> MRIGIISVGPGNIMNLYRGVKRASENFEDVSIELVESPRNDLYDLLFIPGVGHFGEGMRRLRENDLIDFVRKHVEDERYVVGVCLGMQLLFEESEEA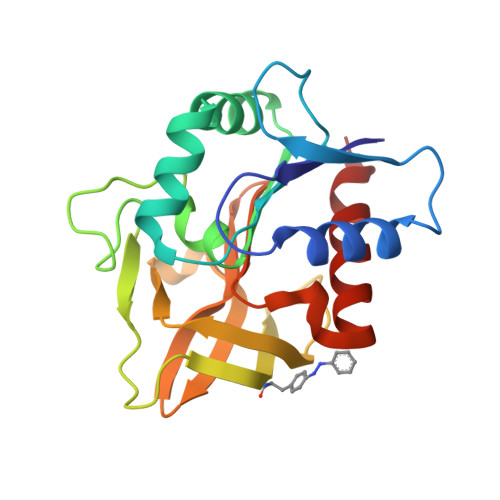PGVKGLSLIEGNVVKLRSRRLPHMGFNEVIFKDTFPNGYYYFVHTYRAVCEEEHVLGTTEYDGEIFPSAVRKGRILGFQFHPEKSSKIGRKLLEKVIECSLSRR>MTIAKDANTFFGAESVQDPYPLYERMRAAGSVHRIANSDFYAVCGWDAVNEAIGRPEDFSSNLTATMTYTAEGTAKPFEMDPLGGPTHVLATADDPAHAVHRKLVLRHLAAKRIRVMEQFTVQAADRLWVDGMQDGCIEWMGAMANRLPMMVVAELIGLPDPDIAQLVKWGYAATQLLEGLVENDQLVAAGVALMELSGYIFEQFDRAAADPRDNLLGELATACASGELDTLTAQVMMVTLFAAGGESTAALLGSAVWILATRPDIQQQVRANPELLGAFIEETLRYEPPFRGHYRHVRNATTLDGTELPADSHLLLLWGAANRDPAQFEAPGEFRLDRAGGKGHISFGKGAHFCVGAALARLEARIVLRLLLDRTSVIEAADVGGWLPSILVRRIERLELAVQ[2x]

P450 monooxygenase enzymes are hemoproteins that typically catalyse the activation of molecular oxygen and the insertion of an atom of oxygen into a substrate bound close to the heme iron. The Mtb gene Rv1777 (CYP144A1) from the pathogenic strain H37Rv (which encodes the cytochrome P450 enzyme CYP144A1) is located in a region of the Mtb genome rich in genes encoding proteins of unknown function. The apparent exclusive conservation of CYP144 P450 family enzymes in the mycobacteria suggests the retention of an important catalytic role. In addition, the CYP144A1 deletion strain was markedly more susceptible to growth inhibition by azole drugs than the wild-type Mtb22. These data point to important function(s) for CYP144A1 in Mtb, and possibly to its participation in the Mtb stress response mechanisms.

The N-terminal truncated version construct of CYP144A1 (CYP144A1-TRV) was generated using the previously prepared full-length version CYP144A1-FLV/pET15b plasmid vector, and by deletion of the region encoding the first 30 amino acids. Consistent with this conclusion, it was found that the CYP144A1-TRV form crystallized readily, allowing the determination of a high resolution (1.55 Å) X-ray structure of the ligand-free CYP144A1-TRV enzyme. The CYP144A1-TRV crystal structure contains two monomers in the asymmetric unit. However, a dimeric solution state is unlikely, since solution state MALLS experiments indicated that both the FLV and TRV forms of CYP144A1 are soluble, monomeric proteins (as are the majority of bacterial P450s). Both monomers in the crystal asymmetric unit have a similar overall conformation, with an rmsd of 0.55 Å for 393 C alpha atoms. The structural elements (F/G-helices and BC-loop region) important in determining active site access and substrate specificity are those that are most distinct in CYP144-TRV from other P450 structures. The relatively long linker region connecting the B-and C-helices folds into an extended beta-hairpin, that occupies the region between the N-terminal beta-sheet and the FG-loop. This creates a large access channel to the heme cavity, approximately 10 Å deep from the protein surface and 10 Å wide. The active site of CYP144A1-TRV is predominantly hydrophobic, with Phe321 and His324 side chains located in close proximity of the heme 6th ligand. These residues are likely to be important in determining substrate selectivity.> GPRSQKQLELKVSELVQFLLIKDQKKIPIKRADILKHVIGDYKDIFPDLFKRAAERLQYVFGYKLVELEPKSNTYILINTLEPVEEDAEMRGDQGTPTTGLLMIVLGLIFMKGNTLKETEAWDFLRRLGVYPTKKHLIFGDPKKLITEDFVRQRYLEYRRIPHTDPVDYEFQWGPRTNLELSKMKVLKFVAKVH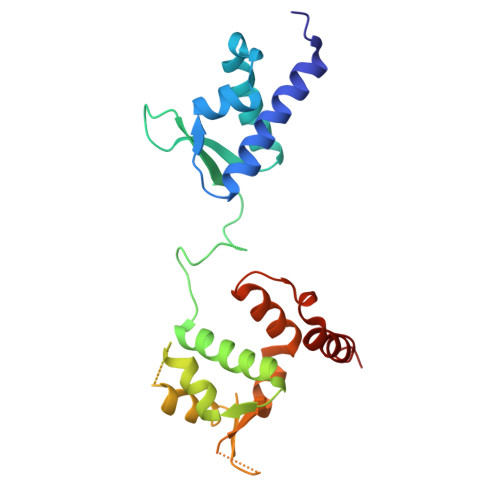NQDPKDWPAQYCEALADEENRAR> IVGGYTCGANTVPYQVSLNSGYHFCGGSLINSQWVVSAAHCYKSGIQVRLGEDNINVVEGNEQFISASKSIVHPSYNSNTLNNDIMLIKLKSAASLNSRVASISLPTSCA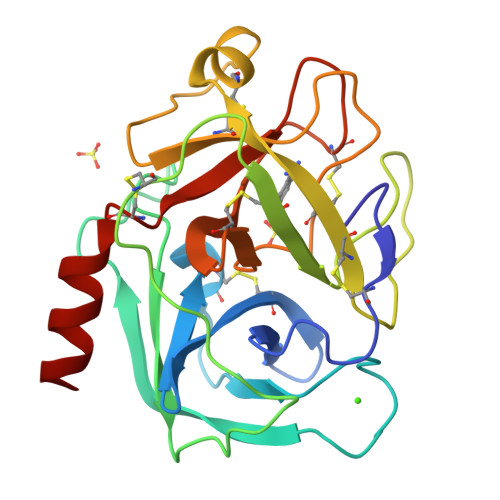SAGTQCLISGWGNTKSSGTSYPDVLKCLKAPILSDSSCKSASSAIITSNMFCAGYLEGGKDSCQGDSGGPVVCSGKLQGIVSWGSGCAQKNKPGVYTKVCNYVSWIKQTIASN> MAELACFCYPHLENDSYKFIPFNNLAIKAMLTAKVDKKDMDKFYDSIIYGIAPPPQFKKRYNTNDNSRGMNFETIMFTKVAMLICEALNSLKVTQANVSNVLSRVVSIRHLENLVIRKENPQDILFHSKDLLLKSTLIAIGQSKEIETTITAEGGEIVFQNAAFTMWKLTYLEHQLMPILDQNFIEYK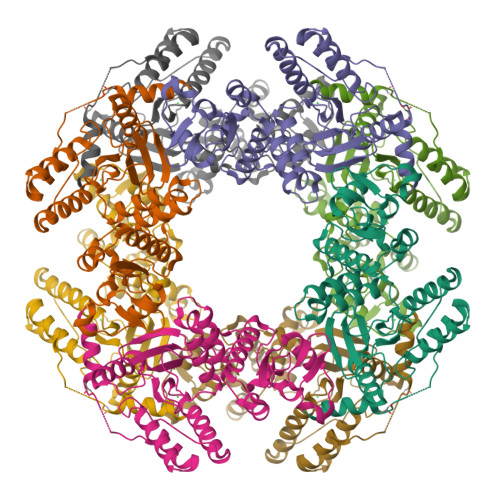VTLNEDKPISDVHVKELVAELRWQYNKFAVITHGKGHYRIVKYSSVANHADRVYATFKSNVKTGVNNDFNLLDQRIIWQNWYAFTSSMKQGNTLDVCKRLLFQKMKPEKNPFKGLSTDRKMDEVAQVGVLVPR>[3x]MHHHHHHENLYFQGAASMSNTTLHATTIYAVRHNGKAAMAGDGQVTLGQQVIMKQTARKVRRLYEGKVLAGFAGSVADAFTLFEKFETKLQQFSGNLERAAVELAQE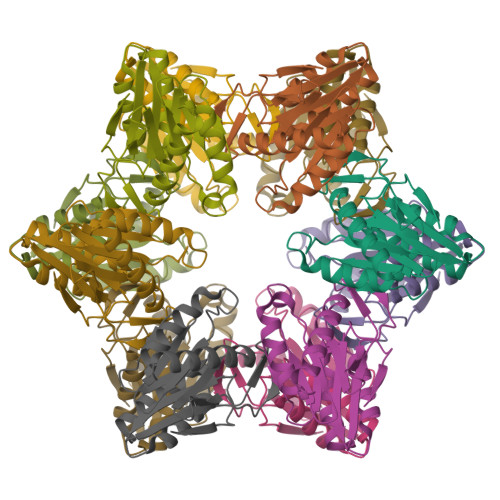WRGDKQLRQLEAMLIVMDKDAILVVSGTGEVIAPDDDLIAIGSGGNYALSAGRALKRHASHLSAEEMAYESLKVAADICVFTNDNIVVETL5-BROMO-2'-DEOXYURIDINE-5'-MONOPHOSPHATE | C9 H12 Br N2 O8 P | 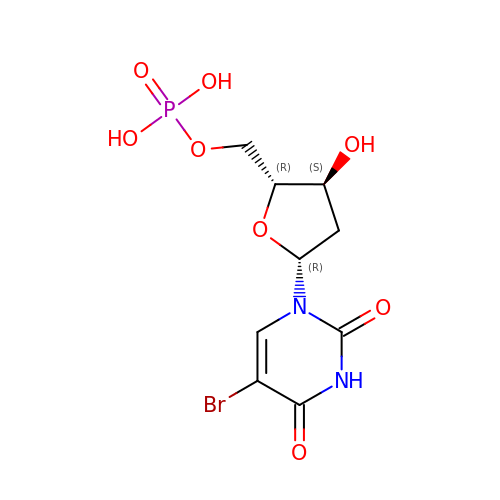LHLHVDBXXZVYJT-RRKCRQDMSA-N>[2x]MKKVLIANRGEIAVRIIRACRDLGIQTVAIYSEGDKDALHTQIADEAYCVGPTLSKDSYLNIPNILSIATSTGCDGVHPGYGFLAENADFAELCEACQLKFIGPSYQSIQKMGIKDVAKAEMIKANVPVVPGSDGLMKDVSEAKKIAKKIGYPVIIKATAGGGGKGIRVARDEKELETGFRMT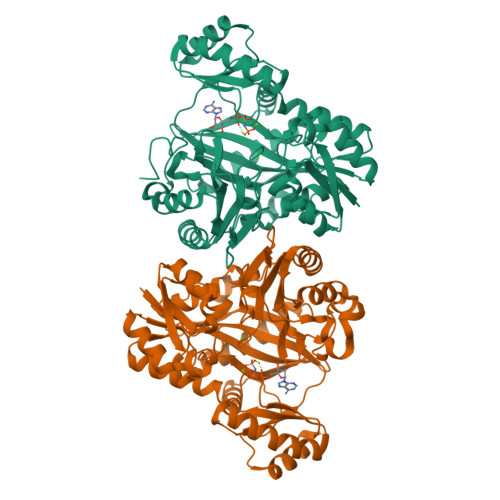EQEAQTAFGNGGLYMEKFIENFRHIEIQIVGDSYGNVIHLGERDCTIQRRMQKLVEEAPSPILDDETRREMGNAAVRAAKAVNYENAGTIEFIYDLNDNKFYFMEMNTRIQVEHPVTEMVTGIDLVKLQLQVAMGDVLPYKQEDIKLTGHAIEFRINAENPYKNFMPSPGKIEQYLAPGGYGVRIESACYTNYTIPPYYDSMVAKLIIHEPTRDEAIMAGIRALSEFVVLGIDTTIPFHIKLLNNDIFRSGKFNTNFLEQNSIMNDEG> ALTEGLGDELEEVIVEKTKQTVASISSGPKHTQKVPILTANETGATMPVLPSDSIETRTTYMHFNGSETDVECFLGRAACVHVTEIQNKDATGIDNHREAKLFNDWKINLSSLVQLRKKLELF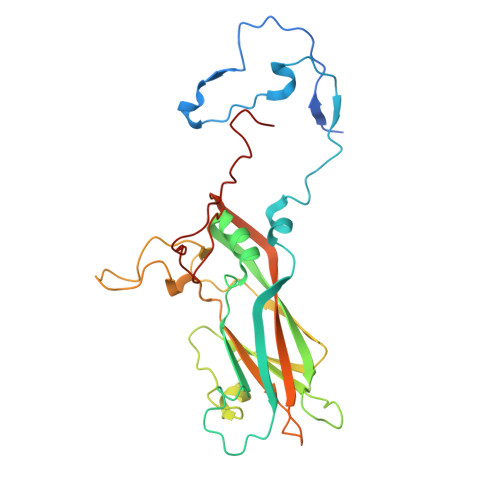TYVRFDSEYTILATASQPDSANYSSNLVVQAMYVPPGAPNPKEWDDYTWQSASNPSVFFKVGDTSRFSVPYVGLASAYNCFYDGYSHDDAETQYGITVLNHMGSMAFRIVNEHDEHKTLVKIRVYHRAKHVEAWIPRAPRALPYTSIGRTNYPKNTEPVIKKRKGDIKSY> GSHMDFVAFMNKINSINANLSRYENIINQIDAQHKDLLTQVSEEQEMELRRSLDDYISQATDLQYQLKADIKDAQRDGLHDSNKQAQAENCRQKFLKLIQDYRIIDSNYK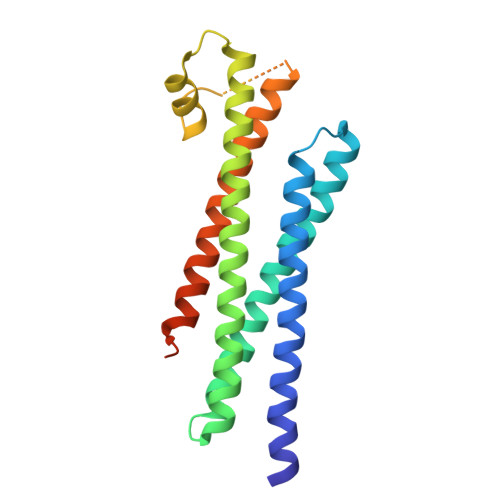EESKEQAKRQYTIIQPEATDEEVEAAINDVNGQQIFSQALLNANRRGEAKTALAEVQARHQELLKLEKTMAELTQLFNDMEELVIELTQLFNDMEELVIE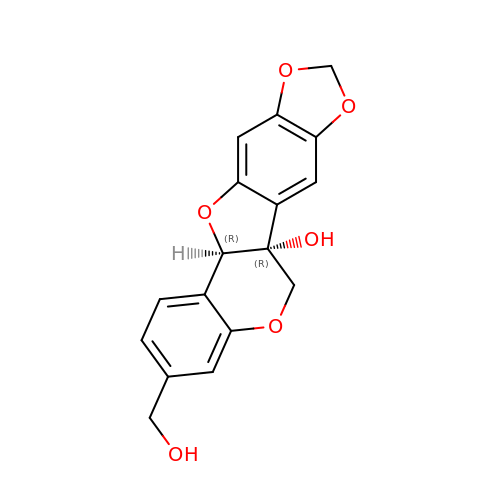(6AR,12AR)-3-(HYDROXYMETHYL)-6H-[1,3]DIOXOLO[5,6][1]BENZOFURO[3,2-C]CHROMEN-6A(12AH)-OL | C17 H14 O6 | JIYYREVJSFXTSG-SJORKVTESA-N> CPGACVCYNEPKVTTSCPQQGLQAVPVGIPAASQRIFLHGNRISHVPAASFRACRNLTILWLHSNVLARIDAAAFTGLALLEQLDLSDNAQLRSVDPATFHGLGRLHTLHLDRCGLQELGPGLFRGLAALQYLYLQDNALQALPDDTFRDLGNLTHLFLHGNRISSVPERAFRGLHSLDRLLLHQNRVAHVHPHAFRDLGRLMT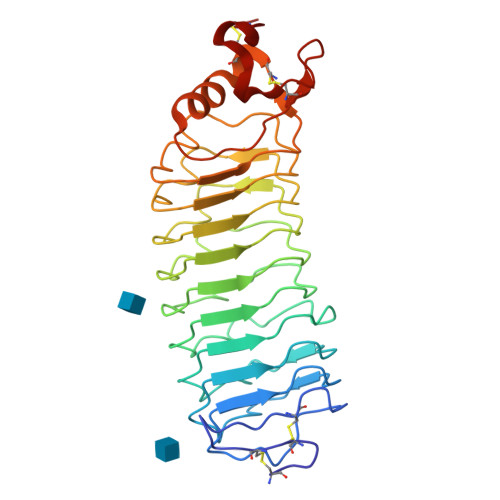LYLFANNLSALPTEALAPLRALQYLRLNDNPWVCDCRARPLWAWLQKFRGSSSEVPCSLPQRLAGRDLKRLAANDLQGCAV>[2x]MPTVSQLQDGLEHPWSLAFLPAEQGLLITERPGRLRLWQQDKGLSPPIAGVPQVYAEGQGGLLEVLPAPDFAASRRVYLSFAEPGEGGKAGTAVGYGRLSDDDARLENFKVIFRQQPKLSVGNHFGGKLAFDRQGYLFIALGENNQRPTAQETDKLQGKLVRLTAEGAVPPDN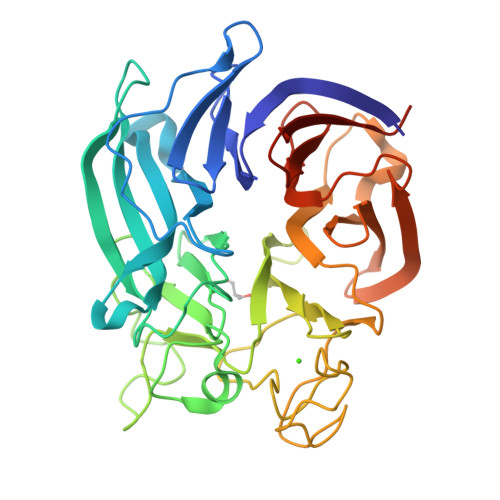PWVGQAGKRPEVWSYGHRNPQGLALNPWSGAIWEHEHGPRGGDELNIPLPGKNYGWPLATYGINYSGQPIPEAKGERVPGTEQPLHYWRVSPGLSGMAFYDGQRFPAWRHSLFIGALAQKALIRLTLEGDKVVAEERLLGDRGERIREVRSGPDGYLYLLTDERDGKLLKVGASLEHHHHHH> MAKDIEISASESKFILEALRQNYRLDGRSFDQFRDVEITFGKEFGDVSVKMGNTKVHCRISCQIAQPYEDRPFEGLFVISTEISPMAGSQFENGNITGEDEVLCSRIIEKSVRRSGALDVEGLCIVAGSKCWAVRADVHFLDCDGGFIDASCIAVMAGLMHFKKPDITVHGEQIIVHPVNEREPVPLGILHIPICVTFSFFNPQDTEENIKGETNSEISIIDATLKEELLRDGVLTVTLNKNREVVQVSKAGGLPMDALTLMKCCHEAYSIIEKITDQILQLLKEDSEKRNKYAAMLTSENAREI;> GHMSRLEIYSPEGLRLDGRRWNELRRFESSINTHPHAADGSSYMEQGNNKIITLVKGPKEPRLKSQMDTSKALLNVSVNITKFSKFERSKSSHKNERRVLEIQTSLVRMFEKNVMLNIYPRTVIDIEIHVLEQDGGIMGSLINGITLALIDAGISMFDYISGISVGLYDTTPLLDTNSLEENAMSTVTLGVVGKSEKLSLLLVEDKIPLDRLENVLAIGIAGAHRVRDLMDEELRKHAQKRVSNASAR;> MAESTTLETIEIHPITFPPEVLARISPELSLQRHLSLGIRPCLRKYEEFRDVAIENNTLSRYADAGNIDTKNNILGSNVLKSGKTIVITSITGGIIEETSASIKDLDDFGEEELFEVTKEEDIIANYASVYPVVEVERGRVGACTDEEMTISQKLHDSILHSRILPKKALKVKAGVRSANEDGTFSVLYPDELEDDTLNETNLKMKRKWSYVLYAKIVVLSRTGPVFDLCWNSLMYALQSVKLPRAFIDERASDLRMTIRTRGRSATIRETYEIICDQTKSVPLMINAKNIAFASNYGIVELDPECQLQNSDNSEEEEVDIDMDKLNTVLIADLDTEAEETSIHSTISILAAPSGNYKQLTLMGGGAKITPEMIKRSLLLSRVRADDLSTRFNI;> GHGNNKEPNTKNRLDSAEKKKKMSVQAEIGILDHVDGSSEFVSQDTKVICSVTGPIEPKARQELPTQLALEIIVRPAKGVATTREKVLEDKLRAVLTPLITRHCYPRQLCQITCQILESGEDEAEFSLRELSCCINAAFLALVDAGIALNSMCASIPIAIIKDTSDIIVDPTAEQLKISLSVHTLALEFVNGGKVVKNVLLLDSNGDFNEDQLFSLLELGEQKCQELVTNIRRIIQDNISPRLVV;> GHMSLSVAEKSYLYDSLASTPSIRPDGRLPHQFRPIEIFTDFLPSSNGSSRIIASDGSECIVSIKSKVVDHHVENELLQVDVDIAGQRDDALVVETITSLLNKVLKSGSGVDSSKLQLTKKYSFKIFVDVLVISSHSHPISLISFAIYSALNSTYLPKLISAFDDLEVEELPTFHDYDMVKLDINPPLVFILAVVGNNMLLDPAANESEVANNGLIISWSNGKITSPIRSVALNDSNVKSFKPHLLKQGLAMVEKYAPDVVRSLENL;> MNVQDRRRLLGPAAAKPMAFSNTTTHVPEKKSTDLTPKGNESEQELSLHTGFIENCNGSALVEARSLGHQTSLISAVYGPRSIRGSFTSQGTISIQLKNGLLEKYNTNELKEVSSFLMGIFNSVVNLSRYPKSGIDIFVYLTYDKDLTNNPQDDDSQSKMTSSQISSLIPHCITSITLALADAGIELVDMAGAGEANGTVVSFIKNGEEIVGFWKDDGDDEDLLECLDRCKEQYNRYRDLMISCLMNQET;> GPHMSTFIFPGDSFPVDPTTPV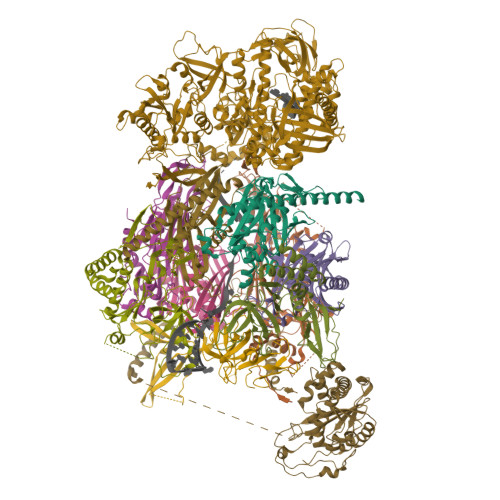KLGPGIYCDPNTQEIRPVNTGVLHVSAKGKSGVQTAYIDYSSKRYIPSVNDFVIGVIIGTFSDSYKVSLQNFSSSVSLSYMAFPNASKKNRPTLQVGDLVYARVCTAEKELEAEIECFDSTTGRDAGFGILEDGMIIDVNLNFARQLLFNNDFPLLKVLAAHTKFEVAIGLNGKIWVKCEELSNTLACYRTIMECCQKNDTAAFKDIAKRQFKEILTVKEE;> RSMSEVITITKRNGAFQNSSNLSYNNTGISDDENDEEDIYMHDVNSASKSESDSQIVTPGELVTDDPIWMRGHGTYFLDNMTYSSVAGTVSRVNRLLSVIPLKGRYAPETGDHVVGRIAEVGNKRWKVDIGGKQHAVLMLGSVNLPGGILRRKSESDELQMRSFLKEGDLLNAEVQSLFQDGSASLHTRSLKYGKLRNGMFCQVPSSLIVRAKNHTHNLPGNITVVLGVNGYIWLRKTSQMDLARDTPSANNSSSIKSTGPTGAVSLNPSITRLEEESSWQIYSDENDPSISNNIRQAICRYANVIKALAFCEIGITQQRIVSAYEASMVYSNVGELIEKNVMESIGSDILTAEKMRGNGN;> GPHMACNFQFPEIAYPGKLICPQYGTENKDGEDIIFNYVPGPGTKLIQYEHNGRTLEAITATLVGTVRCEEEKKTDQEEEREGTDQSTEEEKSVDASPNDVTRRTVKNILVSVLPGTEKGRKTNKYANNDFANNLPKEGDIVLTRVTRLSLQRANVEILAVEDKPSPIDSGIGSNGSGIVAAGGGSGAATFSVSQASSDLGETFRGIIRSQDVRSTDRDRVKVIECFKPGDIVRAQVLSLGDGTNYYLTTARNDLGVVFARAANGAGGLMYATDWQMMTSPVTGATEKRKCAKPF;> GAMSVPAIAPRRKRLADGLSVTQKVFVRSRNGGATKIVREHYLRSDIPCLSRSCTKCPQIVVPDAQNELPKFILSDSPLELSAPIGKHYVVLDTNVVLQAIDLLENPNCFFDVIVPQIVLDEVRNKSYPVYTRLRTLCRDSDDHKRFIVFHNEFSEHTFVERLPNETINDRNNRAIRKTCQWYSEHLKPYDINVVLVTNDRLNREAATKEVESNIITKSLVQYIELLPNADDIRDSIPQMDSFDKDLERDTFSDFTFPEYYSTARVMGGLKNGVLYQGNIQISEYNFLEGSVSLPRFSKPVLIVGQKNLNRAFNGDQVIVELLPQSEWKAPSSIVLDSEHFDVNDNPDIEAGDDDDNNESSSNTTVISDKQRRLLAKDAMIAQRSKKIQPTAKVVYIQRRSWRQYVGQLAPSSVDPQSSSTQNVFVILMDKCLPKVRIRTRRAAELLDKRIVISIDSWPTTHKYPLGHFVRDLGTIESAQAETEALLLEHDVEYRPFSKKVLECLPAEGHDWKAPTKLDDPEAVSKDPLLTKRKDLRDKLICSIDPPGCVDINDALHAKKLPNGNWEVGVHIADVTHFVKPGTALDAEGAARGTSVYLVDKRIDMLPMLLGTDLCSLKPYVDRFAFSVIWELDDSANIVNVNFMKSVIRSREAFSYEQAQLRIDDKTQNDELTMGMRALLKLSVKLKQKRLEAGALNLASPEVKVHMDSETSDPNEVEIKKLLATNSLVEEFMLLANISVARKIYDAFPQTAMLRRHAAPPSTNFEILNEMLNTRKNMSISLESSKALADSLDRCVDPEDPYFNTLVRIMSTRCMMAAQYFYSGAYSYPDFRHYGLAVDIYTHFTSPIRRYCDVVAHRQLAGAIGYEPLSLTHRDKNKMDMICRNINRKHRNAQFAGRASIEYYVGQVMRNNESTETGYVIKVFNNGIVVLVPKFGVEGLIRLDNLTEDPNSAAFDEVEYKLTFVPTNSDKPRDVYVFDKVEVQVRSVMDPITSKRKAELLLK;> GAMASENPDVLLSRVINVVRAASSLASQDVDFYKNLDRGFSKDLKSKADKLADMANEIILSIDEHHESFELKEEDISDLWNNFGNIMDNLLEMSDHSLDKLNCAINSKSRGSDLQYLGEFSGKNFSPTKRVEKPQLKFKSPIDNSESHPFIPLLKEKPNALKPLSESLRLVDDDENNPSHYPHPYEYEIDHQEYSPEILQIREEIPSKSWDDSVPIWVDTSTELESMLEDLKNTKEIAVDLEHHDYRSYYGIVCLMQISTRERDYLVDTLKLRENLHILNEVFTNPSIVKVFHGAFMNIIWLQRDLGLYVVGLFDTYHASKAIGLPRHSLAYLLENFANFKTSKKYQLADWRIRPLSKPMTAYARADTHFLLNIYDQLRNKLIESNKLAGVLYESRNVAKRRFEYSKYRPLTPSSEVYSPIEKESPWKILMYQYNIPPEREVLVRELYQWRDLIARRDDESPRFVMPNQLLAALVAYTPTDVIGVVSLTNGVTEHVRQNAKLLANLIRDALRNIKNTNEEATPIPSSETKADGILLETISVPQIRDVMERFSVLCNSNISKSRAKPVTNSSILLGKILPREEHDIAYSKDGLPNKVKTEDIRIRAQNFKSALANLEDIIFEIEKPLVVPVKLEEIKTVDPASAPNHSPEIDNLDDLVVLKKKNIQKKQPAKEKGVTEKDAVDYSKIPNILSNKPG>[4x]MAAEGVETVSELAPATDKVQNADMAEEDPIFTQLAQKMAAAAEKEEVPVDLLAQYMQVEAHDWHNRVRGAILGLISAVPKVGAAISRLIGLFWPANKVDIWEALRAEEYIRNIVQQELFEFEMRLLENDIQALETTVGRYDTAALTEKGNFLSIWISQADALYIRMRNSTNNIHLLLHMVTVSTLHLAALHERLTFGEELYGTNNSTNWTRDLVDKFETYTSDLIPNVFKRWKEWRPTQIEISAWVRRGSCGNLTCRPDVSYATVEDKISGALFSFQATNRNSTTLFLEVCEDHKTRMVNEAIADMASCLSPTFAFHKLLPDDIQTQFSPYDRQQFGQVFRGPYSQDLSHGLWTAFKNFRSRTTRSDQTLRDRILEVIIRAGHHVDAIQFVYDHSNPNLTTPGTVAGNAAGGTRHQVDVRDRPIQELRME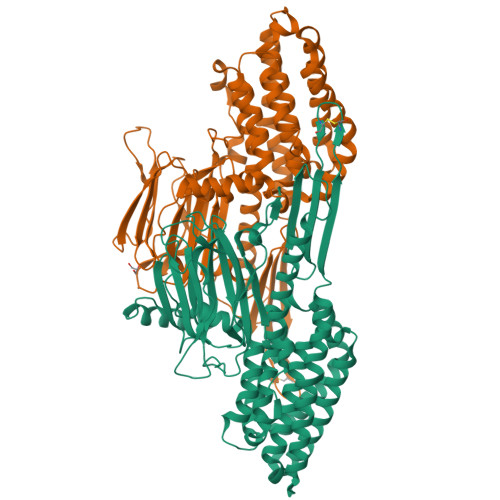FSQDVLASLQLHFEDGTSTRKFGNELGWATRILTCTAPYGYRFSSWAFREDPGPYRTTAISVLRFQFTPELDMPLPASYMLS>HLPRVLKVPATRILLLVLAVIIYGTAGFHFIEGESWTVSLYWTFVTIATVGYGDYSPHTPLGMYFTCTL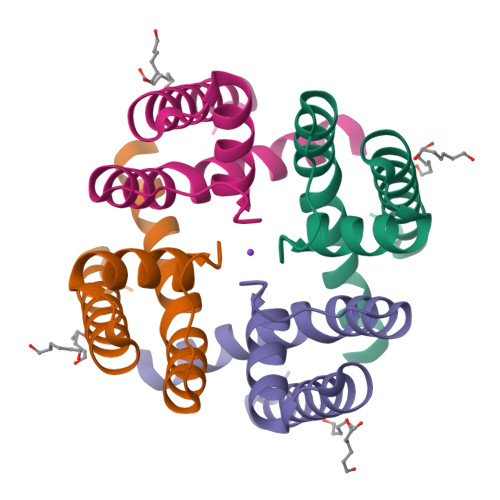IVLGIGTFAVAVERLLEFLINR[8x]In the specialized epithelial tissues, the apical expression of the epithelial sodium channel (ENaC) gives rise to a transepithelial directional flow of Na+ ions. ENaC function is therefore crucial in proper regulation of blood volume and pressure, as well as surface liquid volume in the respiratory and reproductive systems. In the case of ENaC, three homologous subunits, α, β, and γ, form trimers which are arranged in a counterclockwise direction when viewed from the extracellular space. Unlike other ion channels, ENaC activity is primarily modulated by proteases that remove peptidyl tracts in the ECD.

To investigate the structural source of ENaC trimer assembly, we exploited a set of constructs, deemed ENaCFL, which comprises wild-type α and β, and N-terminally eGFP-tagged γ, and behaves like wild-type ENaC as measured by electrophysiology. To determine the structure of ENaCFL, we expressed ENaCFL in HEK293T/17, solubilized in digitonin, and added two different Fabs, 7B1 (recognizes the α subunit) and 10D4 (recognizes the β subunit), to facilitate particle alignment. Reference-free 2D class averages and 3D classifications reveal that ENaCFL channels form as α-β-γ counterclockwise when viewed from outside the cell (Figure 1—figure supplements 2–4). However, the transmembrane domain (TMD) and the cytosolic domain (CD) were not resolved; we speculate that preferred particle orientation, air-water interface denaturation, and intrinsic protein flexibility and conformational heterogeneity contribute to the lack of 3D reconstruction of the TMD and CD. Therefore, we did not include the TMD and CD portions in the ENaCFL structure. We observed a map feature located near the β-ball domain and the β6-β7 loop of the α subunit, where residues αGlu335, αAsp338, and αSer344 in the α-β6-β7 loop have been identified as important in Na+ self-inhibition (Kashlan et al., 2015). The map quality in this region is estimated to be well beyond 3 Å and thus the positions of the side chains are reliable. We speculate that this map feature is a cation, perhaps a Na+ ion, based on the surrounding residues, the above-mentioned functional studies, and the presence of high Na+ (150 mM) during purification. The cation interacts closely with several negative charges: the carboxyl group of αAsp338, and the carbonyl oxygens of αLeu135, αGlu335, and αVal346; all of these interactions are within distances of 2.5 – 3.5 Å. Furthermore, the presence of a phenylalanine adopting a different conformation in the α subunit from the tyrosines in the β and γ subunits, near the cation site confers a specialized function for the α subunit as the primary Na+ sensor.

> MEGNKLEEQDSSPPQSTPGLMKGNKREEQGLGPEPAAPQQPTAEEEALIEFHRSYRELFEFFCNNTTIHGAIRLVCSQHNRMKTAFWAVLWLCTFGMMYWQFGLLFGEYFSYPVSLNINLNSDKLVFPAVTICTLNPYRYPEIKEELEELDRITEQTLFDLYKYSSFTTLVAGSRSRRDLRGTLPHPLQRLRVPPPPHGARRARSVASSLRDNNPQVDWKDWKIGFQLCNQNKSDCFYQTYSSGVDAVREWYRFHYINILSRLPETLPSLEEDTLGNFIFACRFNQVSCNQANYSHFHHPMYGNCYTFNDKNNSNLWMSSMPGINNGLSLMLRAEQNDFIPLLSTVTGARVMVHGQDEPAFMDDGGFNLRPGVETSISMRKETLDRLGGDYGDCTKNGSDVPVENLYPSKYTQQVCIHSCFQESMIKECGCAYIFYPRPQNVEYCDYRKHSSWGYCYYKLQVDFSSDHLGCFTKCRKPCSVTSYQLSAGYSRWPSVTSQEWVFQMLSRQNNYTVNNKRNGVAKVNIFFKELNYKTNSESPSVTMVTLLSNLGSQWSLWFGSSVLSVVEMAELVFDLLVIMFLMLLRRFRSRYWSPGRGGRGAQEVASTLASSPPSHFCPHPMSLSLSQPGPAPSPALTAPPPAYATLGPRPSPGGSAGASSSTCPLGGP;> MHVKKYLLKGLHRLQKGPGYTYKELLVWYCDNTNTHGPKRIICEGPKKKAMWFLLTLLFAALVCWQWGIFIRTYLSWEVSVSLSVGFKTMDFPAVTICNASPFKYSKIKHLLKDLDELMEAVLERILAPELSHANATRNLNFSIWNHTPLVLIDERNPHHPMVLDLFGDNHNGLTSSSASEKICNAHGCKMAMRLCSLNRTQCTFRNFTSATQALTEWYILQATNIFAQVPQQELVEMSYPGEQMILACLFGAEPCNYRNFTSIFYPHYGNCYIFNWGMTEKALPSANPGTEFGLKLILDIGQEDYVPFLASTAGVRLMLHEQRSYPFIRDEGIYAMSGTETSIGVLVDKLQRMGEPYSPCTVNGSEVPVQNFYSDYNTTYSIQACLRSCFQDHMIRNCNCGHYLYPLPRGEKYCNNRDFPDWAHCYSDLQMSVAQRETCIGMCKESCNDTQYKMTISMADWPSEASEDWIFHVLSQERDQSTNITLSRKGIVKLNIYFQEFNYRTIEESAANNIVWLLSNLGGQFGFWMGGSVLCLIEFGEIIIDFVWITIIKLVALAKSLRQRRAQASYAGPPPTVAELVEAHTNFGFQPDTAPRSPNTGPYPSEQALPIPGTPPPNYDSLRLQPLDVIESDSEGDAI;> MAPGEKIKAKIKKNLPVTGPQAPTIKELMRWYCLNTNTHGCRRIVVSRGRLRRLLWIGFTLTAVALILWQCALLVFSFYTVSVSIKVHFRKLDFPAVTICNINPYKYSTVRHLLADLEQETREALKSLYGFPESRKRREAESWNSVSEGKQPRFSHRIPLLIFDQDEKGKARDFFTGRKRKVGGSIIHKASNVMHIESKQVVGFQLCSNDTSDCATYTFSSGINAIQEWYKLHYMNIMAQVPLEKKINMSYSAEELLVTCFFDGVSCDARNFTLFHHPMHGNCYTFNNRENETILSTSMGGSEYGLQVILYINEEEYNPFLVSSTGAKVIIHRQDEYPFVEDVGTEIETAMVTSIGMHLTESFKLSEPYSQCTEDGSDVPIRNIYNAAYSLQICLHSCFQTKMVEKCGCAQYSQPLPPAANYCNYQQHPNWMYCYYQLHRAFVQEELGCQSVCKEACSFKEWTLTTSLAQWPSVVSEKWLLPVLTWDQGRQVNKKLNKTDLAKLLIFYKDLNQRSIMESPANSIEMLLSNFGGQLGLWMSCSVVCVIEIIEVFFIDFFSIIARRQWQKAKEWWAWKQAPPCPEAPRSPQGQDNPALDIDDDLPTFNSALHLPPALGTQVPGTPPPKYNTLRLERAFSNQLTDTQMLDEL>GSHMSQATSQPINFQVQKDGSSEKSHMDDYMQHPGKVIKQNNKYYFQTVLNNASFWKEYKFYNANNQELATTVVNDNKKADTRTINVAVEPGYKSL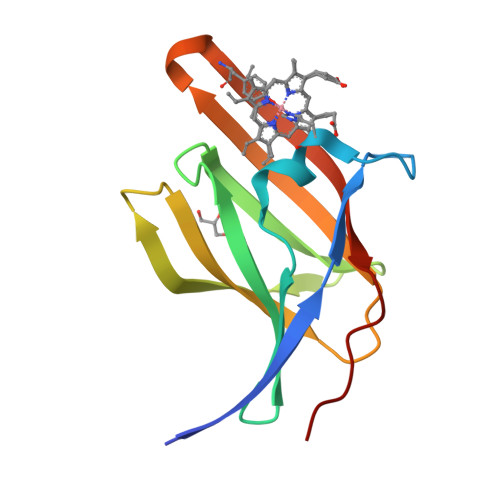TTKVHIVVPQINYNHRYTTHLEFEKAIPTLA[2x]2-(4-phenoxyphenoxy)-6-[(1S,4S)-5-propanoyl-2,5-diazabicyclo[2.2.1]heptan-2-yl]pyridine-3-carboxamide | C26 H26 N4 O4 | 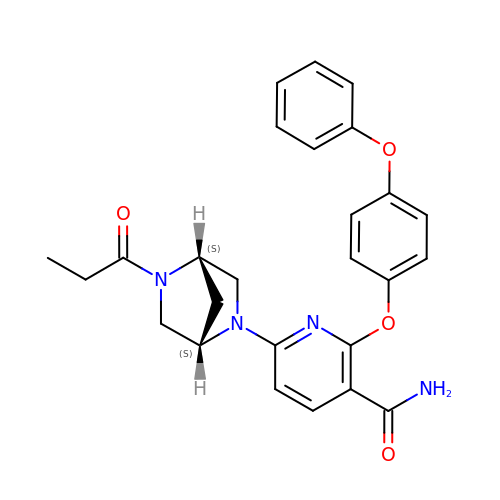DQFJRLJIIQKNPY-ROUUACIJSA-N Clathrin-mediated endocytosis is essential for protein retrieval during neurotransmission and receptor recycling. Accumulation of the adapter proteins at the plasma membrane initiates the endocytic event and contributes to membrane bending. Complex formation has been observed between the ENTH domain of epsin and the ANTH domain of Sla2, the yeast homolog of human huntingtin interacting protein 1 related (Hip1R). Epsin and the phospholipid PIP2 are essential for clathrin-mediated endocytosis, and we show how assemblies are formed between the ENTH domain of epsin and the ANTH domain of Sla2 in fungi.

A crystal structure was determined of a complex between the ENTH domain of Ent2 (ENTH2) from S. cerevisiae and the PIP2 phospholipid to a resolution of 3.4 Å. The structure shows two ENTH2 domains sandwiched around one PIP2 molecule. The inositol head group of PIP2 is bound to the previously identified phosphatidylinositol-binding pocket of one of the ENTH2 molecules. In the second ENTH2 molecule, the N-terminal α0 is unfolded (ENTH2Noα0), and the electron density suggests the N-terminal residues are extended. In the ENTH2/PIP2 structure, the α0 helix points away from the ENTH2 domain and there are no interactions with the phosphoinositol group. As a result of α0 reorientation pointing away from the ENTH2α0 molecule, the second ENTH2Noα0 molecule can form interactions with the phosphatidylinositol head group. However, most of the buried area (1020 Å2) contributed to the dimer interface comes from the α0 helix of the ENTHα0 domain, which is repositioned by the PIP2 molecule to facilitate dimer formation. The effect of PIP2 binding is therefore twofold; it attaches the ENTH domain to the membrane and displaces the α0 helix, so it can form a dimer with a second ENTH domain. In the ENTH2/PIP2 structure, two α0 helices from symmetry-related ENTH2α0 molecules stack against each other to create a homotetramer containing two PIP2 molecules in the same plane, ready to insert into the membrane. We thus conclude that the PIP2/ENTH2 crystal structure shows an intermediate state, where the binding of one PIP2 dimerizes two ENTH2 domains and prepares the “empty” ENTH domain to bind another PIP2.

>[2x]MSKQFVRSAKNMMKGYSSTQVLVRDATANDSRTPSIDTLDDLAQRSYDSVDFFEIMDMLDKRLNDKGKYWRHVAKSLTVLDYLVRFGSENCVLWCRENFYVIKTLREFRHENESGFDEGQIIRVKAKELVSLLNDEERLREERSMNTRNRRANRAA>MDFAYTEEKETIKINNIMIHKYTVLYTSNCIMDIYSEEEKITCFSNRLVFLERGVNISVRMQKQILSEKPYVAFALNGDMLRHLKDALMIIYGMSKIDTNACRSMSRKIMTTEVNKTLLDELKNINSHDNSAFISSLIYLISKLENNEKIIESIYISSVSFFSDKVRNLIEKDLSRKWTLGIIADAFNASEITIRKRLESENTNFNQILMQLRMSKAALLLLENSYQISQISNMIGISS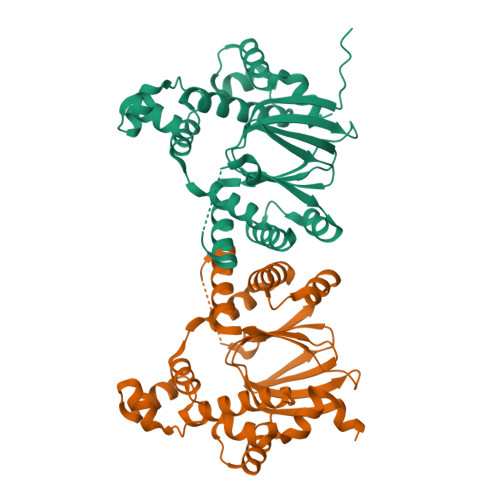ASYFIRIFNKHYGVTPKQFFTYFKGG[2x]An increasing number of surface‐associated proteins identified in Gram‐positive bacteria are characterized by intramolecular cross‐links in structurally conserved thioester, isopeptide, and ester domains (TIE proteins). TEDs are predicted at the distal end of a large number of surface proteins from Gram‐positive bacteria, and the name TIE (thioester, isopeptide, ester) proteins have been introduced for this family. Internal thioester bonds, formed between Cys and Gln side‐chains and first identified in the second thioester domain (TED) of the Streptococcus pyogenes minor pilin Cpa,3 play a negligible role in protein stability, but are suggested to mediate covalent bacterial adhesion. Structures of Bacillus anthracis, vancomycin‐resistant Staphylococcus aureus, and vancomycin‐resistant Enterococcus faecium TEDs show a head domain with Class I topology extended by a β‐sandwich; the latter contributes the thioester bond‐forming Gln via a β‐hairpin insertion into the head domain.

A BaTIE construct (Glu35‐Lys557 of the full, translated open reading frame) was designed to exclude both the N‐terminal Sec secretion signal peptide (Met1‐Ala34), and a 38‐residue C‐terminal region upstream of the LPATG putative sorting motif predicted to be natively unfolded. Its experimental molecular mass (58,441 Da) was determined by ESI‐MS as 70 Da lighter than predicted, consistent with the formation of a single thioester bond (evolving one molecule of ammonia) and three isopeptide bonds (evolving two molecules of ammonia and one water molecule). The crystal structure of BaTIE was determined to 2.58 Å resolution using Se‐SAD phasing and standard refinement approaches. Continuous electron density between the Cys71 and Gln266 side‐chains of BaTIE confirms the presence of a thioester bond in this position, consistent with previous data. Further, continuous electron density between Lys297/Asn373, Lys384/Asp464, and Lys475/Asn555 side‐chains reflects the presence of isopeptide bonds, positioned adjacent to putative catalytic residues Glu343, Glu443, and Glu524, respectively. In both chains of BaTIE in the asymmetric unit (ASU), the electron density for IPD3 gets progressively weaker the farther away from IPD2 the residues are positioned, suggesting flexibility of IPD3 in the crystal. The BaTIE ASU contains seven bound metal ions in three unique sites. The third site is coordinated by Asp142 and Gln144 side‐chains belonging to two neighboring ASUs, and two water molecules. It is likely these are zinc ions derived from the crystallization condition and are unlikely to be biologically significant, given that crystal packing is a prerequisite for co‐ordination. To test collagen binding of BaTIE in its full‐length, enzyme‐linked immunosorbence assays were performed using a BaTIE‐Flag tag fusion. These static adhesion assays strongly suggest that BaTIE does not interact with Collagens I–IV or gelatin.

>GAMEVMNRETYKMDWSYSNSKQREIKTEIIKTASGSIAYCLTPDLRSPNGEDLPEMGKTSDAVYRVLLNGYPQKGPSELGVATTEEAHYATQLAVWIAANELTEEDLVAKNERVHNLMKRLVEASKKETGSQDVFFKVNPVDSQTATQNGDYLETGFYAVQTNAVSGSYTILPENAPKGLRIVNENGEEKSTLSINEKFKILLPKDTSSGNFKMKVKSTLTNLQAIAFKGSEKVQNTTVLLQRNSEKISTDLVVNWESVGSLKIMKLGEKKEVLKGAVFEVSNENFKQNVTTSDKGIAELGNLPIGIYSVKEIQAPAGYVLDRSVKKIEVKTGETAVLELKNENVKGELEITKVDVADGNTKLPNAEFTIYNEQGKEVVKGKTDEKGVAKFKLPYGKYTYKETIAPNGYVINEETFAFEIKENGEIIKHIVQDKKVEGELEITKVDVADGNTKLPNAEFTIYNEQGKEVVKGKTNEQGIAKFKLPYGKYTYKETIAPNGYVINEEKFGFEIKENGEIIKHIVKNKK[2x]>[6x]EGLTIDLKNFRKPGEKTFTQRSRLFVGNLPPDITEEEMRKLFEKYGKAGEVFIHKDKGFGFIRLETRTLAEIAKVELDNMPLRGKQLRVRFACHSASLTVRNLPQYVSNELLEEAFSVFGQVERAVVIVDDRGRPSGKGIVEFSGKPAARKALDRCSEGSF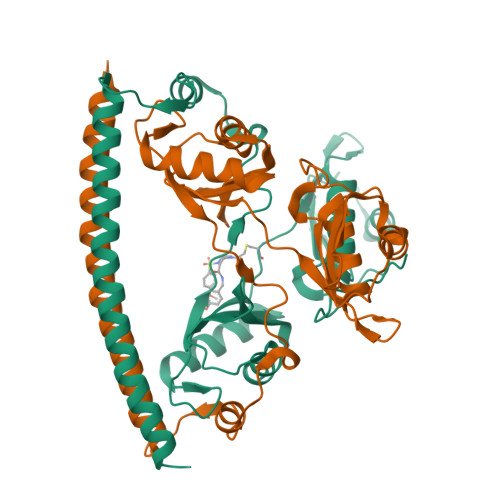LLTTFPRPVTVEPMDQLDDEEGLPEKLVIKNQQFHKEREQPPRFAQPGSFEYEYAMRWKALIEMEKQQQDQVDRNIKEAREKLEMEMEAARHEHQ> CUGCUGCUGCCGC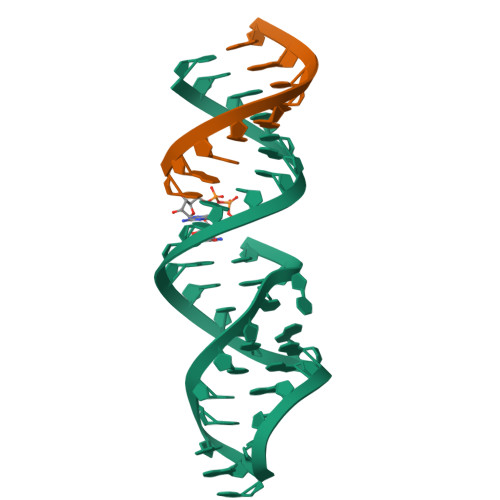UAAGGAUGAAAGUCUAUGC;> CAGCAGCAG N-Acyl homoserine lactonases (AHL-lactonases) have important functions in decreasing pathogenicity by degrading AHLs. Unlike most AHL-lactonases, AidH is proposed to be a member of the α/β-hydrolase fold family. AidH contains a substrate-binding tunnel between the core domain and the cap domain. Taken together, the present results reveal the catalytic mechanism of the metal-independent AHL-lactonase, which is a typical acid–base covalent catalysis.

We also solved the crystal structure of AidHE219G–C6-HS at 1.11 Å resolution. When AidHE219G crystals are soaked with C6-HSL, C6-HSL is degraded to C6-HS, indicating that the AidHE219G mutant does not lose its hydrolytic activity completely. Surprisingly, the mutant AidHE219G is not completely inactive and the activity of AidHY160G is significantly decreased. The absence of the Glu219 side chain causes the backbone of the loop between β7 and α5 to shift by 1 Å. Although the conformational change of His248 reduces the hydrolytic efficiency, AidHE219G is not completely inactive. The biochemical data demonstrate that the Glu219→Gly mutation weakens the His-dependent solvent-assisted deprotonation and thus decreases the activity of AidH. Moreover, the hydroxyl group in the structure of AidHE219G–C6-HS flips to the opposite side compared with that in AidH–C4-­HS and forms a hydrogen bond to Met144 instead of Tyr160. Two possible conformations of the newly formed hydroxyl group are found. The two or three terminal C atoms of the acyl chain in the AidHE219G–C6-HS structure shift by approximately 3 Å compared with AidHS102G–C6-HSL. The low-quality electron density and higher B factor (31.5 Å2) in this region indicate that the AHL tail is relatively flexible.

>[2x]MTINYHELETSHGRIAVRESEGEGAPLLMIHGNSSSGAIFAPQLEGEIGKKWRVIAPDLPGHGKSTDAIDPDRSYSMEGYADAMTEVMQQLGIADAVVFGWSLGGHIGIEMIARYPEMRGLMITGTPPVAREEVGQGFKSGPDMALAGQEIFSERDVESYARSTCGEPFEASLLDIVARTDGRARRIMFEKFGSGTGGNQRDIVAEAQLPIAVVNGRDGPFVELDFVSKVKFGNLWEGKTHVIDNAGHAPFREAPAEFDAYLARFIRDCTQLEHHHHHH>SNAVLVASCSAPSQPSPDSPTTNASSSQTREATTYPLTVDNCGTTATFDS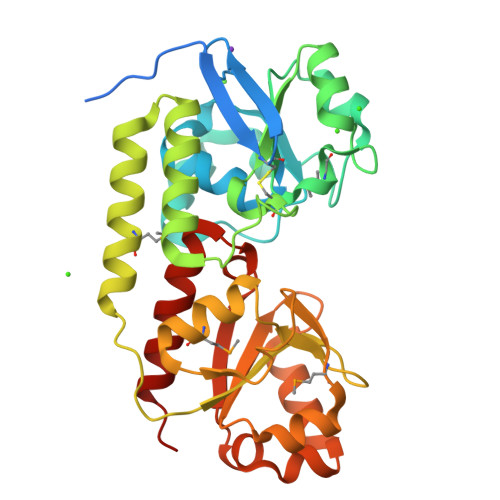VPERVVTLKSSTTELLLALGRGDRIVATSYLDGPVAPWLEDEAAQVPAVSAPLDERLPSLEKVLETEPDLIFAGWESMVTTEGLADRDRLTQLGVNTLVAPSACKEDGYRPDPLTWESLAQEITTVGTIFDAHSEAQSLVDTMNEQLAAISPDSRGLSALWFSSGSDTPFVGGGSGSAQLVMDTVGLRNIGSDIDDTWGPMSWEAIIDANPDVIVLVDSSWSSAQKKKDILTSHPVASTLDAVVNDRYLVIDFPPTEPGVRTADGAVALADQLAALTVED[2x]5-iodanyl-1H-indazole | C7 H5 I N2 | 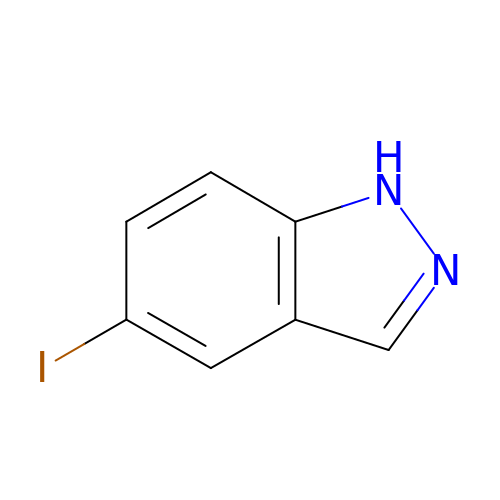CGCHCLICSHIAAM-UHFFFAOYSA-N>[4x]MEGTGVVAVYGNGAITEAKKSPFSVKVGLAQMLRGGVIMDVVNAEQARIAEEAGACAVMALERVPADIRAQGGVARMSDPQMIKEIKQAVTIPV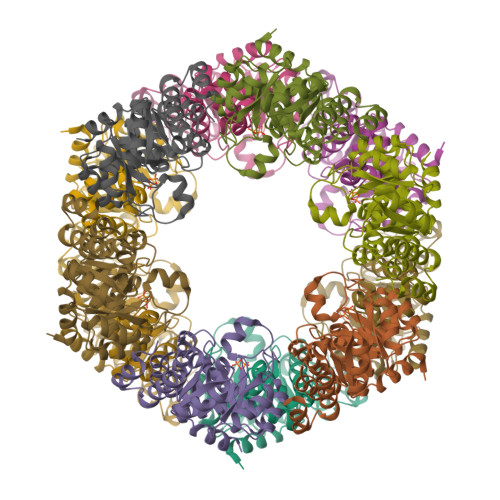MAKARIGHFVEAQILEAIGIDYIDESEVLTLADEDHHINKHNFRIPFVCGCRNLGEALRRIREGAAMIRTRGEAGTGNIIEAVRHVRSVNGDIRVLRNMDDDEVFTFAKKLAAPYDLVMQTKQLGRLPVVQFAAGGVATPADAALMMQLGCDGVFVGSGIFKSGDPARRARAIVQAVTHYSDPEMLVEVSCGLGEAM> MEAGITGTWYNQLGSTFIVTAGADGALTGTYESAVGNAESRY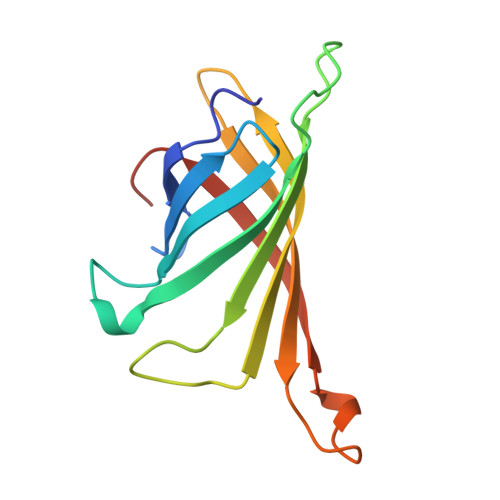VLTGRYDSAPATDGSGTALGWTVAWKNNYRNAHSATTWSGQYVGGAEARINTQWLLTSGTTEANAWKSTLVGHDTFTKVKPSAAS> MAWVTQAYSSGLSQNSIISLTGNDRTVADGTFNSMIMPRAVIANEREHFMKTRIDKIEHDLNRSAKQEMMDRQSLAEDYNALNLAVGQEIKLDIATQHQLNRLGSAMYKADHERETELTDLINRIRENEVTVNGILENQKAITAAERADLLLEVVASTAKSVSAAGRAAADGSGVVPVFGPSVANGIKVGIDIADSVAEAAIAVKESGIITQLNDVYHAFQSVHVAPNDVIKPAAVVAGTSTELIGNLQAIYSRLR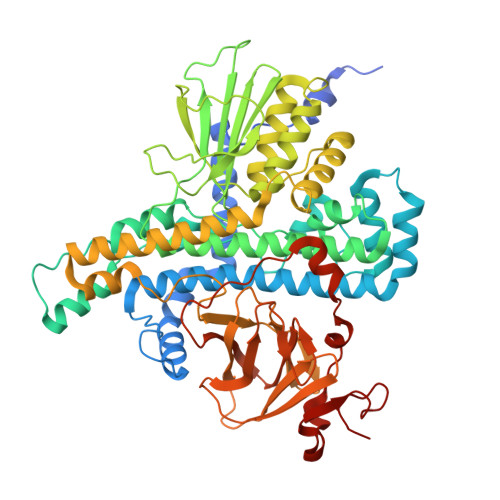SHSDIGFKKATVGDVIPNSYMIKPVNSTEYASWQLYVIHPVQGSLGLVVQLMGDALTYNVFAQYGNTSASEFGKTVLTGGATNTALEGTKVKFQTKVTAQQALALTMALKDAASMLSQGELIGYFEQYINLALEPDNLSLQDNMHKYHHLLTSQNSPIDWNYHDEEMHKWLDSRKTTNYDAMQKKDGTVIADIHIPKVFNDLRNTTLHCKLEGKQTIAGYTVYEYLIGPWAHYGDIDYSVVVDTLNEETKWYCEVIGIDGHLLIEKSVQHKPEKILELTVNDSGVTSFNGRNHDRLKLKVYVKDSLSVKVFRNWIGINAPRVKTKMFNDHIGVKYDYSHFDKNISPAHLTLTDLGWHTWDQYNAGNWTNIKP pentane-1,1-diol | C5 H12 O2 | 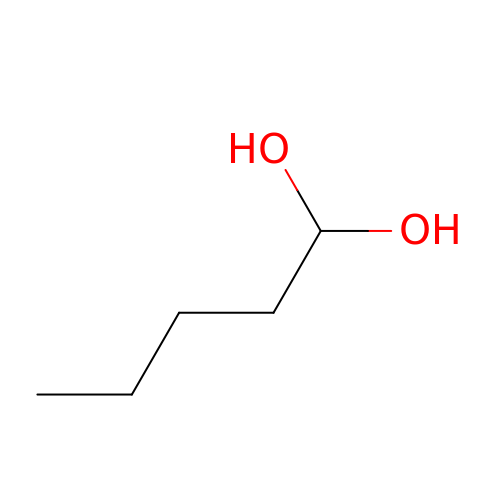UWJJYHHHVWZFEP-UHFFFAOYSA-N> MKESLKDRIRLWKRLYVNAFENALNAIPNVKGVLLAYNTNIDAIKYLDADDLEKRVTEKGKEKVFEIIENPPEKISSIEELLGGILRSIKLGKAMEWFVESEEVRRYLREWGWDELRIGGQAGIMANLLGGVYRIPTIVHVPQNPKLQAELFVDGPIYVPVFEGNKLKLVHPKDAIAEEEELIHYIYEFPRG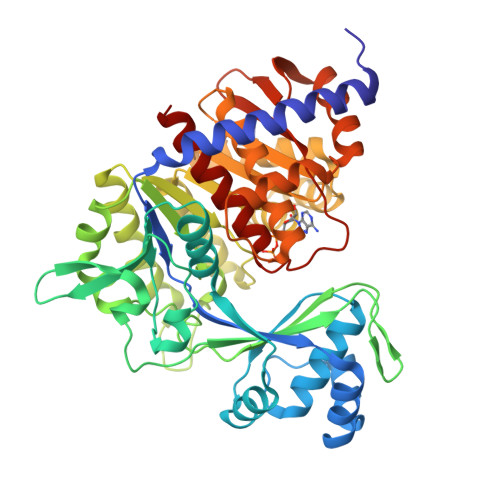FQVFDVQAPRENRFIANADDYNARVYMRREFREGFEEITRNVELAIISGLQVLKEYYPDGTTYKDVLDRVESHLNILNRYNVKSHFEFAYTANRRVREALVELLPKFTSVGLNEVELASIMEIIGDEELAKEVLEGHIFSVIDAMNVLMDETGIERIHFHTYGYYLALTQYRGEEVRDALLFASLAAAAKAMKGNLERIEQIRDALSVPTNERAIVLEEELEKEFTEFENGLIDMVDRQLAFVPTKIVASPKSTVGIGDTISSSAFVSEFGMRKR> ASSTTKCTVSHEVADCSHLKLTQVPDDLPTNITVLNLTHNQLRRLPAANFTRYSQLTSLDVGFNTISKLEPELCQKLPMLKVLNLQHNELSQLSDKTFAFCTNLTELHLMSNSIQKIKNNPFVKQKNLITLDLSHNGLSSTKLGTQVQLENLQELLLSNNKIQALKSEELDIFANSSLKKLELSSNQIKEFSPGCFHAIGRLFGLFLNNVQLGPSLTEKLCLELANTSIRNLSLSNSQLSTTSNTTFLGLKWT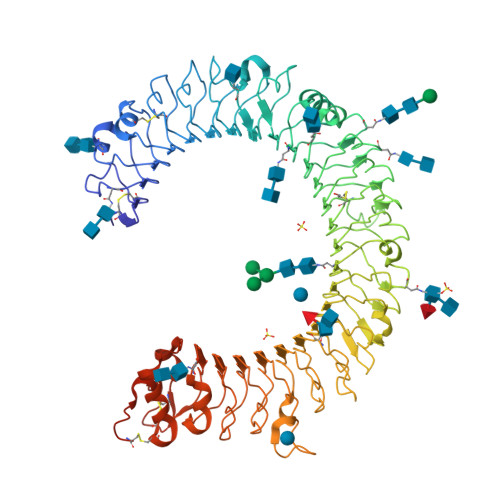NLTMLDLSYNNLNVVGNDSFAWLPQLEYFFLEYNNIQHLFSHSLHGLFNVRYLNLKRSFTKQSISLASLPKIDDFSFQWLKCLEHLNMEDNDIPGIKSNMFTGLINLKYLSLSNSFTSLRTLTNETFVSLAHSPLHILNLTKNKISKIESDAFSWLGHLEVLDLGLNEIGQELTGQEWRGLENIFEIYLSYNKYLQLTRNSFALVPSLQRLMLRRVALKNVDSSPSPFQPLRNLTILDLSNNNIANINDDMLEGLEKLEILDLQHNNLARLWKHANPGGPIYFLKGLSHLHILNLESNGFDEIPVEVFKDLFELKIIDLGLNNLNTLPASVFNNQVSLKSLNLQKNLITSVEKKVFGPAFRNLTELDMRFNPFDCTCESIAWFVNWINETHTNIPELSSHYLCNTPPHYHGFPVRLFDTSSCKDSAPFEENLYFQGDYKDDDDKGSHHHHHH> KPRIDMHSHFFPRISEQEAAKFDANHAPWLQVSAKGDTGSIMMGKNNFRPVYQALWDPAFRIEEMDAQGVDVQVTCATPVMFGYTWEANKAAQWAERMNDFALEFAAHNPQRIKVLAQVPLQDLDLACKEASRAVAAGHLGIQIGNHLGDKDLDDATLEAFLTHCANEDIPILVHPWDMMGGQRMKKWMLPWLVAMPAETQLAILSLILSGAFERIPKSLKICFGHGGGSFAFLLGAVDNAWRHRDIVREDCPRPPSEYVDRFFVDSAVFNPGALELLVSVMGEDRVMLGSDYPFPLGEQKIGGLVLSSNLGESAKDKIISGNASKFFNIN;> KPRIDMHSHFFPRISEQEAAKFDANHAPWLQVSAKGDTGSIMMGKNNFAPVYQALWDPAFRIEEMDAQGVDVQVTCATPVMFGYTWEANKAAQWAERMNDFALEFAAHNPQRIKVLAQVPLQDLDLACKEASRAVAAGHLGIQIGN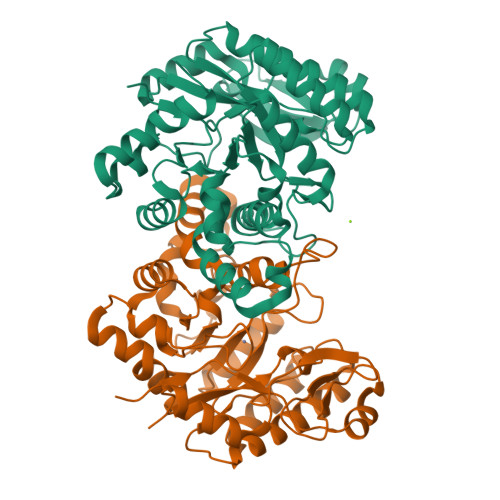HLGDKDLDDATLEAFLTHCANEDIPILVHPWDMMGGQRMKKWMLPWLVAMPAETQLAILSLILSGAFERIPKSLKICFGHGGGSFAFLLGRVDNAWRHRDIVREDCPRPPSEYVDRFFVDSAVFNPGALELLVSVMGEDRVMLGSDYPFPLGEQKIGGLVLSSNLGESAKDKIISGNASKFFNIN>[12x]MERELPIPVFLTEDEDSVHERMLSNFQDVSTLEGDFIYDATRPTAEQIAELKQLGLQNNLKIAFPQTSYGTYLEWLGECKGVFKNQPTKATGVITFTGVQGTIITKGTIVTTIATDEKQSIEFELLETKTIGENETVDIKAESRIVGTIGNVSKGSISVLLGSISGVKSITNKEDFRGGTDIEDEEHFRERVLVAEQEDKLSGASSDYIRWAKEVDGVGYAYVVSEWAGAGTVKVLILDKNRKAATQELIDKVQEYIYPLNISEGENRDGKAPIGALVTVVTPDTLLINVKASFIFSNGFSEETVLNNLKTKIDKYLDKIDLGGTVSYNAIQAIVGSMMLTDEGIEDFSNLTINDVKENIKLQDQVVGIGEIVNEVVG;>MIASKKGKEMLLTLSPIYEQSIIMQSLYEAIGSEFDNLELLDEEIELQLFPQSATWGLGFWENRVGLITNLDEDMETRRRKVIAKLQSKYIMTPKRMSMILQSYTGANIKINENISPYTFGVELTSTQGFPKDLEDLYKRVNVIKPSHLAVSYKLVSLLKSKTYFAQTAIMSEEITIYPYTSKEVKASVKAKFALAHNMSSETLTVYPR[6x];>[6x]MVIDIYLKNEKEKIDFHFPVNPQDSLSIKKEKRFETVDIVNLGEFDIKKEGEKIREISFKTFLPNLYDASYCRYSELKNPIEVVAMLEKWVDQAEPLRLIITGFGYNGLVTISSFSNTQTAGREEDRDIEITFRTYRELKIETLKKDTKSNTKTDLKDNRPNTQTKSKIYTVKASDTLYKIAKNLLGKGSRWPEIYNIPENKKVIGKNPNIIKKGQKLVIPSK;>[6x]MYNDDYIEEASFLNGSDVVILIDGVEELYMEEIKADFEQDEQSIKLLGCQNEISRVGTTKGSFSLNGYKTDSKFAKLGFRSFEIIYNLSNSETLGYESIRLKNCRLKKLPLINSKAGEIVKIEVEGSFRGYDLLNEL;>MATGTWNEKERKEIPGFYNRFKTQAEKSTNTGLKGRLAMPIRANWGDVGKVVTIKNDLRQLKNLFGDDMNYSAFKLGKLALLGNVKELLLYRLVDGNQKKGTLTLKDTTENSAKDVIKLETKYPTARNFNVTIKSNLVDSDKKDFIFFENTKQLFSSSIKGTIDEIVLEINSNLDNEYVIATKVADSDTILANVVNQALEGGNDGCTSITNESYLKALEEFERYSFDSFVLDGVADEALQETTKAWVAKNKELGKDILLFLGGKTEDNIKQINDKSKSFNDENIVNVGSSAYYENIKYTPSEVAVYIAALSVSKGITGSICNAKTIFEEVEPRLSQSEVKECLKSGTLVLDFDDGDVIIVDDVNTFKKYVDDKNEAMGYISNIMFINTINKDTSLKRKEFVGKIFNDATGQTTVICALKKYFEELMSQGIISEFNVDIDTELQATAKADEFYWKWDAVKVDVMKKIYGTGYLG[6x];>[6x]MPNLFPQSETFETVELKNNDENELDLKGSFLFDFEKGEFVKNADGTLKKCDKVQAYKQWCQKAILTPRYKKAAYTNIYGSEIKDLIASNLSQSAKELEITRLIKETILVHPYTKEVGEFSFNWLENSRLVEYEFDVLTIDDENIVIDGNIKR

Here, we reveal the extended and contracted atomic structures of an intact contractile-tailed phage (φCD508) that binds to and penetrates the protective S-layer of the Gram-positive human pathogen Clostridioides difficile. The virion can be divided into five distinct regions: the head, neck, tail, baseplate, and needle. Structures of purified φCD508 virions in both extended and contracted conformations were determined by single-particle EM of frozen-hydrated samples; the resolution ranged from 2.6 to 4.0 Å for the extended phage, and 2.9 to 4.2 Å for the contracted form.

The tail is terminated by the baseplate. Importantly, the baseplate of φCD508 must be adapted for binding and penetration of the host cell S-layer. The baseplate is minimal compared with other structurally characterized phages consisting of only six unique proteins. These are organized into a baseplate hub, which connects to the tail, and a wedge, which forms a collar around the needle. The baseplate is also expected to include the host attachment proteins gp67 and gp68, constituting the tail fiber and receptor binding proteins that bind to the C. difficile S-layer. Although these could not be sufficiently resolved in the EM maps for atomic modeling, low-pass–filtered maps show protrusions for the tail fibers. The association of domain III with the triplex protein gp65a wing domain increases the order of the region such that good density is present for domain III. Peptidoglycan hydrolases that facilitate enzymatic penetration of the cell wall are a common feature of phage baseplates, including in the recent structure of a diffocin, a native C. difficile tailocin. It is striking that we find no obvious auxiliary domains with structural homology to peptidoglycan hydrolases in any of the φCD508 baseplate or needle proteins built to near completion within our cryoEM maps.>AATYAQTLQNIPETNVTTLDNGLRVASEESSQPTCTVGVWIGAGSRYENEKNNGAGYFVEHLAFKGTKKRPCAAFEKEVESMGAHFNGYTSREQTAFYIKALSKDMPKVVELLADVVQNCALEESQIEKERGVILQELKEMDNDMTNVTFDYLHATAFQGTALARTVEGTTENIKHLTRADLASYIDTHFKAPRMVLAAAGGISHKELVDAARQHFSGVSFTYKEDAVPILPRCRFTGSEIRARDDALPVAHVALAVEGPGWADPDNVVLHVANAIIGRYDRTFGGGKHLSSRLAALAVEHKLCHSFQTFNTSYSDTGLFGFHFVADPLSIDDMMFCAQGEWMRLCTSTTESEVKRAKNHLRSAMVAQLDGTTPVCETIGSHLLNYGRRISLEEWDSRISAVDARMVRDVCSKYIYDKCPALAAVGPIEQLLDYNRIRSGMYWIRF[2x];>SLKVAPKVAVSAAAERVKLCPGAEDLEITKLPNGLIIASLENFSPASRIGVFIKAGSRYETTANLGTAHLLRLASPLTTKGASSFRITRGIEAVGGSLSVYSTREKMTYCVECLRDHVDTVMEYLLNVTTAPEFRPWEVTDLQPQLKVDKAVAFQSPQVGVLENLHAAAYKTALANPLYCPDYRIGKITSEQLHHFVQNNFTSARMALVGIGVKHSDLKQVAEQFLNIRSGAGTSSAKATYWGGEIREQNGHSLVHAAVVTEGAAVGSAEANAFSVLQHVLGAGPLIKRGSSVTSKLYQGVAKATTQPFDASAFNVNYSDSGLFGFYTISQAAHAGEVIRAAMNQLKAAAQGGVTEEDVTKAKNQLKATYLMSVETAQGLLNEIGSEALLSGTHTAPSVVAQKIDSVTSADVVNAAKKFVSGKKSMAASGDLGSTPFLDEL[2x];>[2x]MAPNIRKSHPLLKMINNSLIDLPAPSNISAWWNFGSLLAVCLMTQILTGLLLAMHYTADTSLAFSSVAHTCRNVQYGWLIRNLHANGASFFFICIFLHIGRGLYYGSYLYKETWNTGVILLLTLMATAFVGYVLPWGQMSFWGATVITNLFSAIPYIGHTLVEWAWGGFSVDNPTLTRFFALHFLLPFAIAGITIIHLTFLHESGSNNPLGISSDSDKIPFHPYYSFKDILGLTLMLTPFLTLALFSPNLLGDPENFTPANPLVTPPHIKPEWYFLFAYAILRSIPNKLGGVLALAASVLILFLIPFLHKSKQRTMTFRPLSQTLFWLLVANLLILTWIGSQPVEHPFIIIGQMASLSYFTILLILFPTIGTLENKMLNY;>[2x]GELELHPPAFPWSHGGPLSALDHSSVRRGFQVYKQVCSACHSMDYVAFRNLIGVTHTEAEAKALAEEVEVQDGPDENGELFMRPGKISDYFPKPYPNPEAARAANNGALPPDLSYIVNARHGGEDYVFSLLTGYCDPPAGVVVREGLHYNPYFPGQAIGMAPPIYNEILEYDDGTPATMSQIAKDVCTFLRWAAEPEHDQRKRMGLKMLLISALLTSLLYYMKRHKWSVLKSRKMAYRPPK;>VHNDVTVPDFSAYRREDVMDATTSSQTSSEDRKGFSYLVTATACVATAYAAKNVVTQFISSLSASADVLALSKIEIKLSDIPEGKNVAFKWRGKPLFVRHRTQAEINQEAEVDVSKLRDPQHDLDRVKKPEWVILVGVCTHLGCVPIANSGDFGGYYCPCHGSHYDASGRIRKGPAPYNLEVPTYQFVGDDLVVVG[2x];>AARATVAGGGRLMDRIRKWYYNAAGFNKYGLMRDDTLYEDDDVKEALKRLPEDLYNERMFRIKRALDLSLKHRILPKEQWVKYEEDKPYLEPYLKEVIRERLEREAWNKK[2x];>[2x]GIHFGNLARVRHIITYSLSPFEQRAIPNIFSDALPNVWRRFSSQVFKVAPPFLGAYLLYSWGTQEFERLKRKNPADYENDQ;>LRGSGEEEEEELVDPLTTIREHCEQTEKCVKARERLELC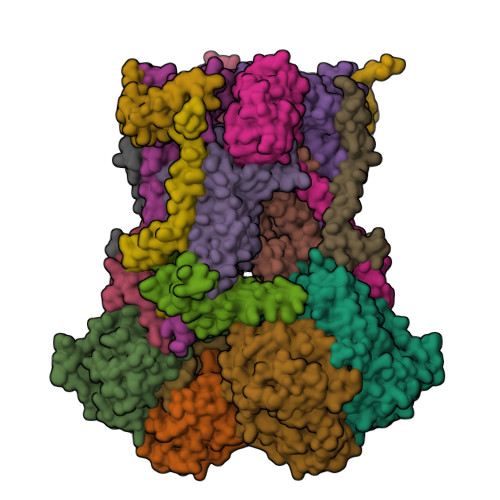DARVSSRSHTEEQCTEELFDFLHARDHCVAHKLFNKLK[2x];>ALLRQAYSALFRRTSTFALTVVLGAVLFERAFDQGADAIFEHLNEGKLWKHIKHKYEASEE[2x]>S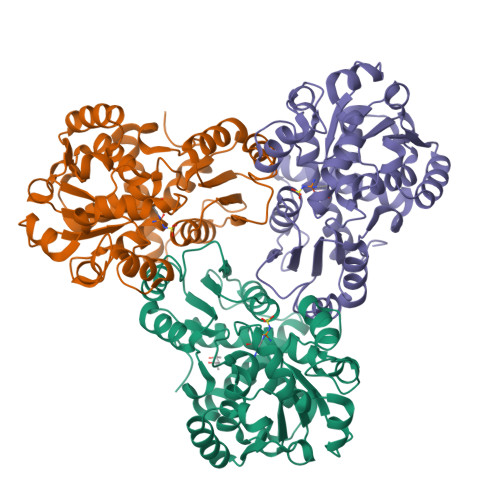GFYHKHFLKLLDFTPAELNSLLQLAAKLKADKKSGKEEAKLTGKNIALIFEKDSTRTRCSFEVAAYDQGARVTYLGPSGSQIGHKESIKDTARVLGRMYDGIQYRGYGQEIVETLAEYASVPVWNGLTNEFHPTQLLADLLTMQEHLPGKAFNEMTLVYAGDARNNMGNSMLEAAALTGLDLRLVAPQACWPEAALVTECRALAQQNGGNITLTEDVAKGVEGADFIYTDVWVSMGEAKEKWAERIALLREYQVNSKMMQLTGNPEVKFLHCLPAFHDDQTTLGKKMAEEFGLHGGMEVTDEVFESAASIVFDQAENRMHTIKAVMVATLSK[3x]[4-[[4-(ethylamino)-5-(trifluoromethyl)pyrimidin-2-yl]amino]-2-fluoranyl-5-methoxy-phenyl]-morpholin-4-yl-methanone | C19 H21 F4 N5 O3 | 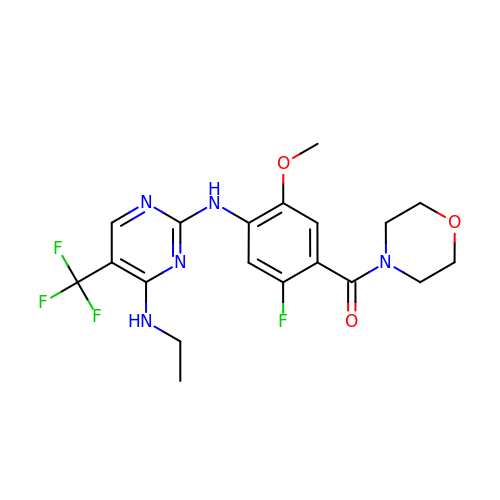XCFLWTZSJYBCPF-UHFFFAOYSA-N>[2x]ETGIEGRKPTCDEKYANIT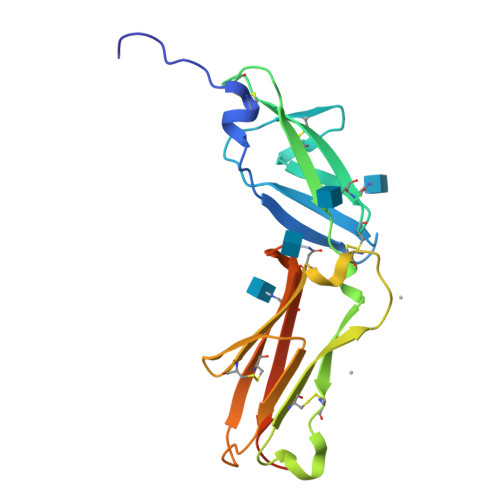VDYLYNKETKLFTAKLNVNENVECGNNTCTNNEVHNLTECKNASVSISHNSCTAPDKTLILDVPPGVEKFQLHDCTQVEKADTTICLKWKNIETFTCDTQNITYRFQCGNMIFDNKEIKLENLEPEHEYKCDSEILYNNHKFTNASKIIKTDFGSPGEGTKHHHHHH Regnase-1 (also known as Zc3h12a and MCPIP1) is an RNase whose expression level is stimulated by lipopolysaccharides and prevents autoimmune diseases by directly controlling the stability of mRNAs of inflammatory genes such as interleukin (IL)-6, IL-1β, IL-2, and IL-12p404567. Regnase-1 accelerates target mRNA degradation via their 3′-terminal untranslated region (3′UTR), and also degrades its own mRNA8. Regnase-1 is a member of Regnase family and is composed of a PilT N-terminus like (PIN) domain followed by a CCCH-type zinc–finger (ZF) domain, which are conserved among Regnase family members. Our findings suggest that Regnase-1 cleaves its target mRNA by an NTD-activated functional PIN dimer, while the ZF increases RNA affinity in the vicinity of the PIN dimer.

X-ray crystallography was attempted for the fragment containing both the PIN and ZF domains, however, electron density was observed only for the PIN domain, consistent with a previous report on Regnase-1 derived from Homo sapiens. This suggests that the PIN and ZF domains exist independently without interacting with each other. We found that the PIN domain formed a head-to-tail oligomer that was commonly observed in all three crystal forms in spite of the different crystallization conditions. In contrast, our gel filtration data, mutational analyses, and NMR spectra all indicate that the PIN domain forms a head-to-tail dimer in solution in a manner similar to the crystal structure. The previously reported crystal structure of the Regnase-1 PIN domain derived from Homo sapiens is nearly identical to the one derived from Mus musculus in this study, with a backbone RMSD of 0.2 Å. The importance of residues W182 and R183 can readily be understood in terms of the monomeric PIN structure as they are located near to the RNase catalytic site; however, the importance of residue K184, which points away from the active site is more easily rationalized in terms of the oligomeric structure, in which the “secondary” chain’s residue K184 is positioned near the “primary” chain’s catalytic site. In contrast, R214 is important for oligomerization of the PIN domain and the “secondary” chain’s residue R214 is also positioned near the “primary” chain’s active site within the dimer interface. Within the crystal structure of the PIN dimer, the Regnase-1 specific basic regions in both the “primary” and “secondary” PINs are located around the catalytic site of the primary PIN. Based on these observations, we concluded that PIN-PIN dimer formation is critical for Regnase-1 RNase activity in vitro.

>[2x]GPHMDLRPVVIDGSNVAMSHGNKEVFSCRGILLAVNWFLERGHTDITVFVPSWRKEQPRPDVPITDQHILRELEKKKILVFTPSRRVGGKRVVCYDDRFIVKLAFESDGVVVSNDTYRDLQGERQEWKRFIEERLLMYSFVNDKFMPPDDPLGRHGPSLDNFLRKKPLPSEHRKQPCPYGKKCTYGIKCRFFHPERPSRPQRSVADELRA> MIFSVDAVRADFPVLSREVNGLPLAYLDSAASAQKPSQVIDAEAEFYRHGYAAVHAGAHTLSAQATEKMENVRKRASLFINARSAEELVFVRGTTEGINLVANSWGNSNVRAGDNIIISQMEHHANIVPWQMLCARVGAELRVIPLNPD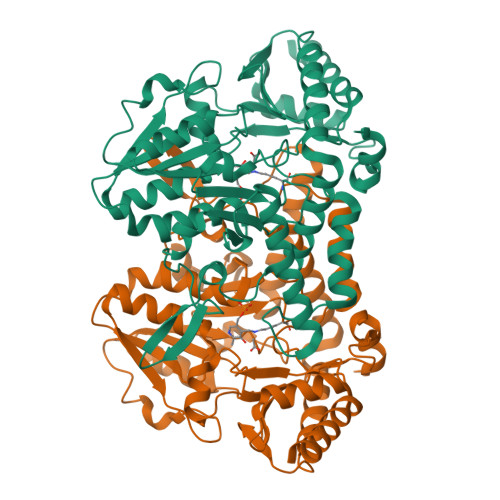GTLQLETLPTLFDAATRLLAITHVSNVLGTENPLAEMITLAHQHGAKVLVDGAQAVMHHPVDVQALDCDFYVFSGHKLYGPTGIGILYVKEALLQEMPPWEGGGSMIATVSLSEGTTWTKAPWRFEAGTPNTGGIIGLGAALEYVSALGLNNIAEYEQNLMHYALSQLESVPDLTLYGPQARLGVIAFNLGAHHAYDVGSFLDNYGIAVRTGHHCAMPLMAYYNVPAMCRASLAMYNTHEEVDRLVTGLQRIHRLLG>[4x]TRDFNGTWEMESNENFEGWMKALDIDFATRKIAVRLTFTEVIDQDGDNFKTKATSTFWNYDVDFTVGVEFDEYTKSLDN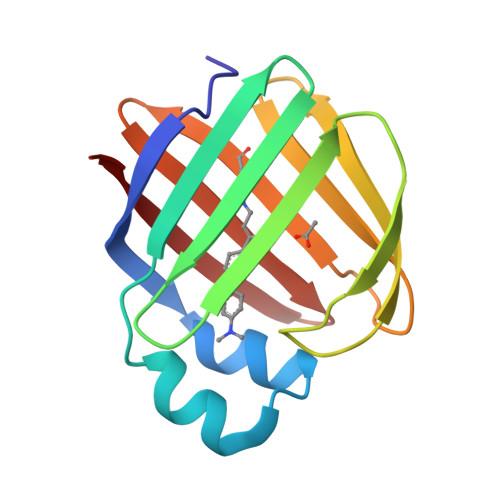RHVKALVTWEGDVLVCVQKGEKENRGWKKWIEGDKLYLELTCGDQVCRQVFKKK> MSNIKINDVFQRIQYAASAGQTQFTIPFPFFDNEYVLVWQNGVQLVMGGAPGQYGISGAGSPSGGLITLVTPAALNDIITIQGDMPIDRTSIYSATISNLTGSDLNGDFNREVVMMKQIQTTQALLQLQYAPWLEVSQDPDVTKDRYLPLLGSGQVWRMNDSGTGIEAYTIDETPAPSSSPFIIYQADATLSNAQNLG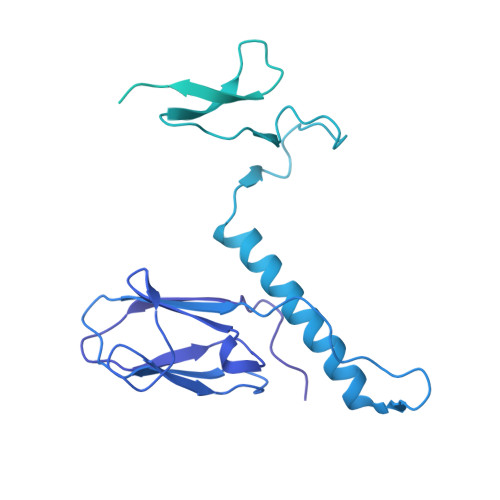ALTSGILKQTVGGGSSTLSIAQNAVDYWAPGDELTRSQAPVSPDDVVNKAYADSIASGFTFINPVNAASTANFNSTYNNGSSGVGATLTATSNGAFSLDGQAGVLNKSYLMKDQTNTFENGIYILTQVGDGSTPAILTRATYFDQPSEIQPGDLVPVLAGTVNNGTLWLQTDTVSAVGTDPITFIAFLPAFSNIVTISGNQTITGDKTFTGTTTLDNFIFVGSNIQHLGDTGNQIIFGTATQINTINNNTISDLSSSGLRLGAANARVSTILDEDDMASDSATALATQQSIKAYVDNFRAAGAILQTVSTNMTNTFSASLAAGSGFSDVTGFNVSITPSATANKVFIKVDMLLASDTVDIVVVVRLKRNGTPIDIGNAAGSRIQITTGSTNAKALDGLQAVSFSFLDSPATTSAITYQVDIGQRTSGSAVGIVVNRSGADVDSSSYTRGASTITAQEIKG> SNAMKRLPLLAA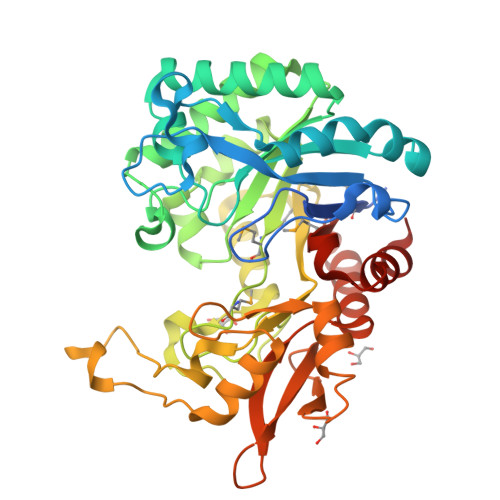LPLLCASALSAQPLMSVGYFNGGGDVTAGPGGDIDKLDVRQITHLNYSFGLIYNDEKDETNAALKDPAHLHEIWLSPKVQADLQKLPALRKQNPDLKVLLSVGGWGARGFSGAAATAESRAVFIRSAQKIIQQYGLDGIDLDWEFPVNGAWGLVASQPADRDNFTALLKSLREAVGEQKLVTIAVGANAESPKSWVDVKAVAPVLNYINLMTYDMAYGTQYFNSNLYDSSHWPTVAAADKYSADFVVNNYLAAGLKPSQMNLGIGFYGRVPKRAVEPGIDWTKADAQNNPVTQPYFGPQQIALFASLGYDLSKDTYVKYNDIVGKLLNDPQKRFTEHWDDEAKVPWLSVQSAEGKPLFALSYENPRSVAIKADYIKAKGLAGAMFWEYGADDQNQLARQLAESLGIKH>MVDFKLSPSQLEARRHAQAFANTVLTKASAEYSTQKDQLSRFQATRPFYREAVRHGLIKAQVPIPLGGTMESLVHESIILEELFAVEPATSITIVATALGLMPV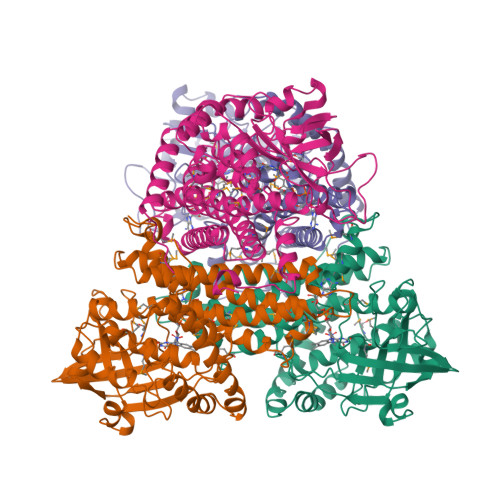ILCDSPSLQEKFLKPFISGEGEPLASLMHSEPNGTANWLQKGGPGLQTTARKVGNEWVISGEKLWPSNSGGWDYKGADLACVVCRVSDDPSKPQDPNVDPATQIAVLLVTRETIANNKKDAYQILGEPELAGHITTSGPHTRFTEFHVPHENLLCTPGLKAQGLVETAFAMSAALVGAMAIGTARAAFEEALVFAKSDTRGGSKHIIEHQSVADKLIDCKIRLETSRLLVWKAVTTLEDEALEWKVKLEMAMQTKIYTTDVAVECVIDAMKAVGMKSYAKDMSFPRLLNEVMCYPLFDGGNIGLRRRQMQRVMALEDYEPWAATYGSSKVDKSRL[4x]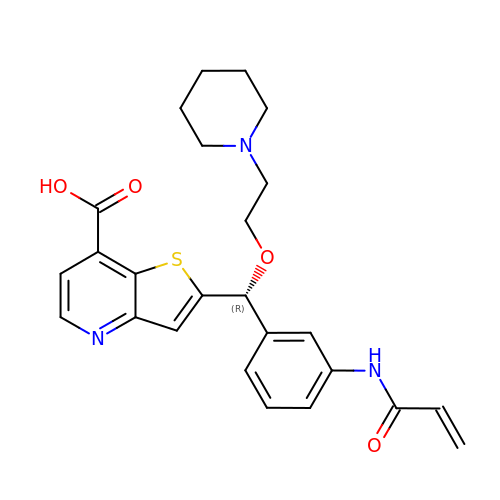2-{(R)-[3-(acryloylamino)phenyl][2-(piperidin-1-yl)ethoxy]methyl}thieno[3,2-b]pyridine-7-carboxylic acid | C25 H27 N3 O4 S | GFSKHNOSSPZNTP-HSZRJFAPSA-N The bacterial injectisome, or type III secretion system (T3SS), is a specialized syringe-shaped protein-export system utilized by many pathogenic Gram-negative bacteria for the injection of virulence proteins (effectors) into host cells. The injectisome can be divided into three major regions: the inner- (IM) and outer-membrane (OM) spanning basal body with associated export apparatus and ATPase components, an extracellular needle, and a terminating pore inserted into the host cell membrane called the translocon. The major structural scaffold of the basal body is comprised largely of three proteins that arrange into a series of highly oligomerized, concentric rings: two intimately associated proteins localized to the IM - PrgK/EscJ/MxiJ and PrgH/EscD/MxiG, and a third protein belonging to the secretin family of OM proteins, InvG/EscC/MxiD (Salmonella enterica serovar Typhimurium SPI-1, Enteropathogenic Escherichia coli (EPEC) LEE and Shigella dysenteriae nomenclature, respectively). In summary, we report the crystal structures for the cytoplasmic and periplasmic domains of PrgH and InvG, two of the main basal body components of the prototypical Salmonella SPI-1 injectisome.

For both the cytoplasmic and periplasmic domains of PrgH, we applied a 24-mer oligomerization constraint, according to the established stoichiometry. For the periplasmic domain, we observed that in preliminary modelling runs, residues 361–369 moved during the local perturbation step, and led to a model with a diameter not supported by the EM map, and relatively poor correlation. We therefore performed the docking procedures using residues 173–361, which led to a model with excellent correlation to the EM map. The model of the IM PrgH periplasmic ring is broadly similar to previously reported models from our groups and others. Importantly, our PrgH periplasmic domain model possesses fully refined interfaces. For the periplasmic domain of PrgH, we engineered numerous interface and surface mutations. Notably, we identified a loop (residues 319–324) that mediates several side- and main-chain contacts with the adjacent subunit. Side-chain mutations within this loop (K320L, T324L) have no effect on secretion; however, mutation of the conformationally labile Gly322 to a leucine abrogates secretion (middle), suggesting that the loop main chain conformation/contacts are more critical to interface integrity. However, mutant variant G322Y in the periplasmic domain of PrgH, or Q97L in InvG, disrupts needle complex assembly. Finally, analysis of the surface electrostatics of the InvG and PrgH periplasmic ring models reveals an acidic surface present on the face of the InvG ring proximal to PrgH, and a complementary basic surface on the corresponding face of PrgH.

>LDSLLGQEKERFQVLPGRDKMLYVAAQNERDTLWARQVLARGDYDKNARVINENEENKRISIWLDTYYPQLAYYRIHFDEPRKPVFWLSRQRNTMSKKELEVLSQKLRALMPYADSVNITLMDDVTAAGQAEAGLKQQALPYSRRNHKGGVTFVIQGALDDVEILRARQFVDSYYRTWGGRYVQFAIELKD[24x]>[2x]MSGADRSPNAGAAPDSAPGQAAVASAYQRFEPRAYLRNNYAPPRGDLCNPNGVGPWKLRCLAQTFATGEVSGRTLIDIGSGPTVYQLLSACSHFEDITMTDFLEVNRQELGRWLQEEPGAFNWSMYSQHACLIEGKGECWQDKERQLRARVKRVLPIDVHQPQPLGAGSPAPLPADALVSAFCLEAVSPDLASFQRALDHITTLLRPGGHLLLIGAL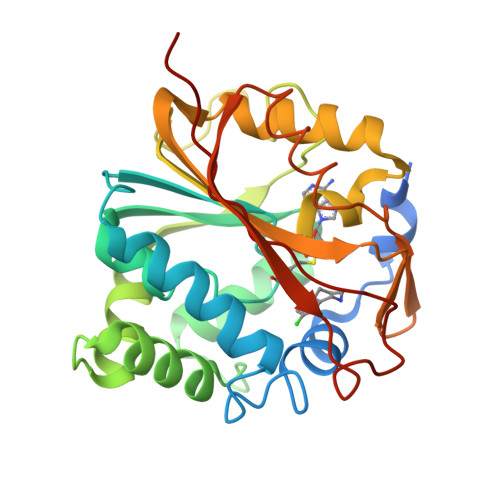EESWYLAGEARLTVVPVSEEEVREALVRSGYKVRDLRTYIMPAHLQTGVDDVKGVFFAWAQKVGL The mitochondrial AAA (ATPase Associated with diverse cellular Activities) protein ATAD1 (in humans; Msp1 in yeast) removes mislocalized membrane proteins, as well as stuck import substrates from the mitochondrial outer membrane, facilitating their re-insertion into their cognate organelles and maintaining mitochondria’s protein import capacity. ATAD1 is a member of a large family of proteins called the AAA (ATPase Associated with diverse cellular Activities) proteins. Six ATAD1 subunits rotate and translocate progressively to form a hexameric spiral assembly. Each ATAD1 subunit consists of two subdomains, a large subdomain followed by a small subdomain, and the nucleotide is bound at the interface between the two.

To obtain a homogenous sample for structural analysis, we expressed human ATAD1 lacking the first 40 amino acids (consisting of the transmembrane helix) with an N-terminal His-tag and bearing a commonly used ‘Walker B’ mutation that inactivates ATP hydrolysis but retains ATP binding (Δ40-ATAD1E193Q). Δ40-ATAD1E193Q formed oligomers as assessed by size exclusion chromatography. We took the fraction corresponding to hexamers and incubated it with ATP before preparing samples for cryo-EM imaging. 3D classification of the particles resulted in two distinct hexameric structures. In the first structure, the six ATAD1 subunits (M1–M6) are arranged in a right-handed spiral with an open seam between the top and the bottom subunits (45, 003 particles analyzed), an arrangement resembling the ‘open state’ structure of Msp1, as well as other related AAA proteins (Cooney et al., 2019; Han et al., 2020; Su et al., 2017; Sun et al., 2017; Twomey et al., 2019; Zehr et al., 2017). Refinement of this structure resulted in a map with an average resolution of 3.7 Å. In the ‘open state’, all six subunits adopt similar overall structures. In the next step of translocation, M6 continues to move upward, assuming the M1 position (top position) in the open spiral, detaching fully from M5, which now becomes the new M6, occupying the bottom position. Consequently, the angle between the two subdomains of M5 widens, and the subunit resumes its original conformation as it reaches the M6 position. Upon building all of ATAD1’s amino acids into the EM density, we observed a piece of density in the central pore that resembles a linear peptide in both the closed and the open state structures. The side chain density was clearly visible, and we modeled the peptide as a 10-mer polyalanine.

>MGSSHHHHHHSSGLVPRGSGSDPTRKQKVEAQKQAEKLMKQIGVKNVKLSEYEMSIAAHLVDPLNMHVTWSDIAGLDDVITDLKDTVILPIKKKHLFENSRLLQPPKGVLLYGPPGCGKTLIAKATAKEAGCRFINLQPSTLTDKWYGESQKLAAAVFSLAIKLQPSIIFIDQIDSFLRNRSSSDHEATAMMKAQFMSLWDGLDTDHSCQVIVMGATNRPQDLDSAIMRRMPTRFHINQPALKQREAILKLILKNENVDRHVDLLEVAQETDGFSGSDLKEMCRDAALLCVREYVNSTSEESHDEDEIRPVQQQDLHRAIEKMKKSKDAAFQNVLTHVCLD[6x]> DQSAKEAIEAALADFVKVYNSKDAAGVASKYMDDAAIFPLDMAPVDGRQNIQKLWQGLMDMGVSEPKFTTLNVQKSGDFAFESGSFSLKGPGKDSKLVDIAGIYVEVWRKGQDG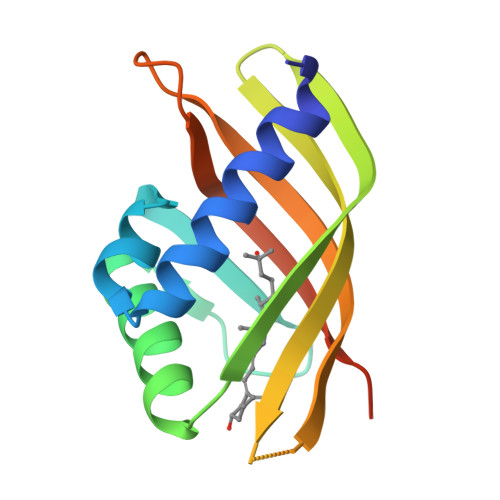GWKLYRTIANLDPAKLEHHHHHH MerTK, a TAM receptor, regulates macrophage efferocytosis and polarization, and its inhibition holds potential for tumor growth suppression and immune modulation. Additionally, MerTK plays a prominent role in regulating efferocytosis, the process by which macrophages engulf and clear apoptotic cells. MerTK is activated upon binding to its ligands, Protein S or growth arrest-specific 6 (GAS6), which recognize phosphatidylserine (PtdSer) exposed on the surface of apoptotic cell debris. In this study, we present a novel strategy for designing MerTK-selective inhibitors by modulating the conformational dynamics of its αC helix.

Since 11 demonstrates highest selectivity with SI of 46.1 among these synthesized inhibitors, the cocrystal structure of MerTK in complex with 11 was resolved to investigate its binding mechanism and molecular basis of the selectivity. The headgroup of 11 orients upward to target the αC helix, while the N,N-dimethylethanamine moiety forms a salt bridge with D678 in the hinge region. This upward binding of 11 contrasts with the previously resolved structures1 and 6which exhibit a downward orientation that extends into the allosteric pocket. Furthermore, the upward positioning of 11 allows the 1-fluorobenzene moiety to form hydrophobic interactions with F634 and A638 on the αC helix and V669 on the β-sheet. Additionally, the para-fluorine of 1-fluorobenzene forms a C–F···O interaction with F634. The acetamide linker forms a hydrogen bond with the backbone of D741, locking MerTK in a DFG-out conformation. Moreover, upon the binding to 11, αC helix of MerTK becomes more stable and adopts an outward conformation in both monomers whereas αC helix is more dynamic and adopts two different conformations upon the binding to 1 or 6. The electron density is also clear and more continuous for αC helix, adjacent β3-αC loop and P-loop, indicating 11 stabilizes αC helix and its surrounding areas. However, in the MerTK/11 structure, the introduction of the longer N,N-dimethylethanamine substitution on Ring-6 results in the shift of adjacent DFG motif to accommodate this longer tail. The differential stabilization of the αC helix by 11 in MerTK versus Tyro3 is consistent with their respective inhibitory effects, with IC50 values of 21.5 nM for MerTK and 991.3 nM for Tyro3. These findings suggest that the selectivity of 11 for MerTK over Tyro3 is attributed to its interactions with and stabilization of the αC helix of MerTK.

>EELQNKLEDVVIDRNLLILGKILGEGEFGSVMEGNLKQEDGTSLKVAVKTMKLDNSSQREIEEFLSEAACMKDFSHPNVIRLLGVCIEMSSQGIPKPMVILPFMKYGDLHTYLLYSRLETGPKHIPLQTLLKFMVDIALGMEYLSNRNFLHRDLAARNCMLRDDMTVCVADFGLSKKIYSGDYYRQGRIAKMPVKWIAIESLADRVYTSKSDVWAFGVTMWEIATRGMTPYPGVQNHEMYDYLLHGHRLKQPEDCLDELYEIMYSCWRTDPLDRPTFSVLRLQLEKLLESLPDV[2x]> LGSENDVIELDDVANIMFYGEGEVGDNHQKFMLIFDTGSANLWVPSKKCNSSGCSIKNLYDSSKSKSYEKDGTKVDITYGSGTVKGFFSKDLVTLGHLSMPYKFIEVIDTDDLEPIYSSVEFDGILGLGWKDLSIGSIDPIVVELKNQNKIDNALFTFYLPVHDVHAGYLTIG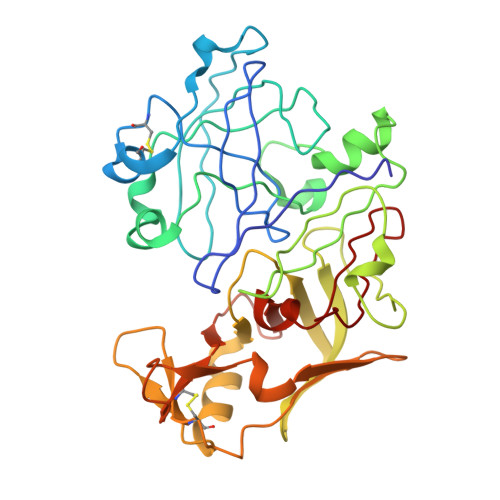GIEEKFYEGNITYEKLNHDLYWQIDLDVHFGKQTMEKANVIVDSGTTTITAPSEFLNKFFANLNVIKVPFLPFYVTTCDNKEMPTLEFKSANNTYTLEPEYYMNPILEVDDTLCMITMLPVDIDSNTFILGDPFMRKYFTVFDYDKESVGFAIAKN> GKLPEEELKKKIEEFANFFIENKDVDLDELADKILEIAEETGTHIGDIYEQLVALAPDEETLRTLTLALVRLLGRRKEPLDLDLVRLLVETLVLDLGATDLAVEVVKLAFSLAKKKEQLEKLLKAI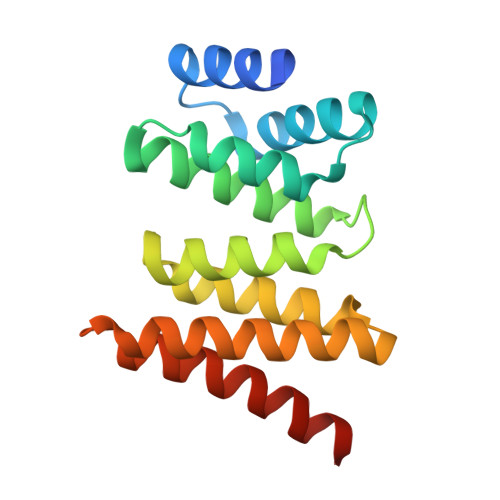DEVIEKARKEKGMDAAAEKLREVKEKYLLEHHHHHH>[2x]MEKYNPHAIEAKWQRFWEEKGFMKAKDLPGGRGKQYVLVMFPYPSGDLHMGHLKNYTMGDVLARFRRMQGYEVLHPMGWDAFGLPAENAALKFGVHPKDWTYANIRQAKESLRLMGILYDWDREVTTCEPEYYRWNQWIFLKMWEKGLAYRAKGLVNWCPKCQTVLANEQVVEGRCWRHEDTPVEKRELEQWYLRITAYAERLLKDLEGLNWPEKVKAMQRAWIGRSEGAEILFPVEGKEVRIPVFTTRPDTLFGATFLVLAPEHPLTLELAAPEKREEVLAYVEAAKRKTEI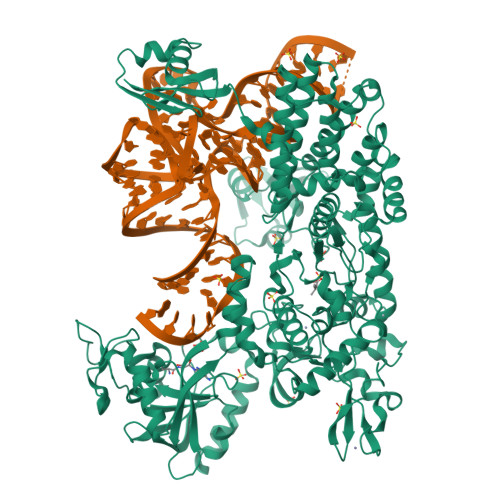ERQAEGREKTGVFLGAYALNPATGERIPIWTADYVLFGYGTGAIMAVPAHDQRDYEFARKFGLPIKKVIERPGEPLPEPLERAYEEPGIMVNSGPFDGTESEEGKRKVIAWLEEKGLGKGRVTYRLRDWLISRQRYWGTPIPMVHCEACGVVPVPEEELPVLLPDLKDVEDIRPKGKSPLEAHPEFYETTCPKCGGPAKRDTDTMDTFFDSSWYYLRYTDPHNDRLPFDPEKANAWMPVDQYIGGVEHAVLHLLYSRFFTKFLHDLGMVKVEEPFQGLFTQGMVLAWTDFGPVEVEGSVVRLPEPTRIRLEIPESALSLEDVRKMGAELRPHEDGTLHLWKPAVMSKSKGNGVMVGPFVKEQGADIARITILFAAPPENEMVWTEEGVQGAWRFLNRIYRRVAEDREALLETSGVFQAEALEGKDRELYGKLHETLKKVTEDLEALRFNTAIAALMEFLNALYEYRKDRPVTPVYRTAIRYYLQMLFPFAPHLAEELWHWFWPDSLFEAGWPELDEKALEKDVVEVAVQVNGRVRGTIHIPKDAPLEVARAEALKVRNVRAHLEGKEVVKEIYVPGKILNLVVRG>[2x]LPAKENEGCIVSVNSGKRYCLPVGQRSGYSLPDWIVGQEVYVDSGAKAKVLLSDWD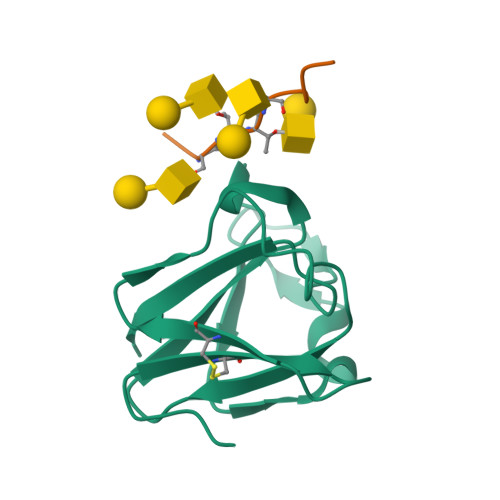NLSYNRIGEFVGNVNPADMKKVKAWNGQYLDFSKPRSMRVVYK;>AASTTTPAPAX[2x]At present, the best structurally characterized pLGIC is the G. violaceus ligand-gated ion channel (GLIC), of prokaryotic origin. Each subunit consists of an extracellular domain (ECD), predominantly in a β-sandwich fold, and a transmembrane domain (TMD) composed of four helices, labeled M1–M4. However, the GLIC is a pH-gated channel, activated by lowering the pH, with a maximal activation at pH 4 and a pH50 around 5. We instead found that proton activation is a complex multiple loci mechanism, with the key contribution stemming from the coupling interface between the extracellular and transmembrane domain, with E35 acting as a key proton-sensing residue.

In the lower part of the ECD, the principal (+) face also carries two acidic residues, E82 and D115. E82Q and D115N display significantly higher proton sensitivity than E82A and D115A, respectively. Assuming that Gln and Asn faithfully mimic protonated side chains of Glu and Asp, this would suggest that residues E82 and D115 are also proton sensors. To investigate this idea, the structures of E82Q and E82A were solved at pH 4. The E82A structure is similar to that of the Wt pH 4 structure, whereas that of E82Q shows a marked local reorganization of the Q82 moiety. Assuming E82 to be in a protonated state at pH 4, Gln is not a good mimic of a protonated Glu residue because Q82 is engaged in a completely different set of interactions with neighboring residues. Therefore, the E82Q mutant phenotype is likely due to local side chain reorganizations of Y28 and F156 rather than being a proton sensor itself. There are no significant differences, measured as 5-fold over Wt, seen in the backbone Cα residues of any of the resolved structures, with the exception of E35A and E82Q. The E82Q side chain takes on a different rotamer, causing a local change in the backbone, as well as a cascading rotamer/conformational change in Y28 and F156, the latter of which flips out towards the aqueous environment. All structures were in the apparently open conformation.

>[5x]GQDMVSPPPPIADEPLTVNTGIYLIECYSLDDKAETFKVNAFLSLSWKDRRLAFDPVRSGVRVKTYAPEAIWIPEIRFVNVENARDADVVDISVSPDGTVQYLERFSARVLSPLDFRRYPFDSQTLHIYLIVRSVDTRNIVLAVDLEKVGKNDDVFLTGWDIESFTAVVKPANFALEDRLESKLDYQLRISRQYFSYIPNIILPMLFILFISWTAFWSTSYEANVTLVVSTLIAHIAFNILVETNLPKTPYMTYTGAIIFMIYLFYFVAVIEVTVQHYLKVESQPARAASITRASRIAFPVVFLLANIILAFLFFGF>[2x]MPALDLIRPSVTAMRVIASVNADFARELKLPPHIRSLGLISADSDDVTYIAA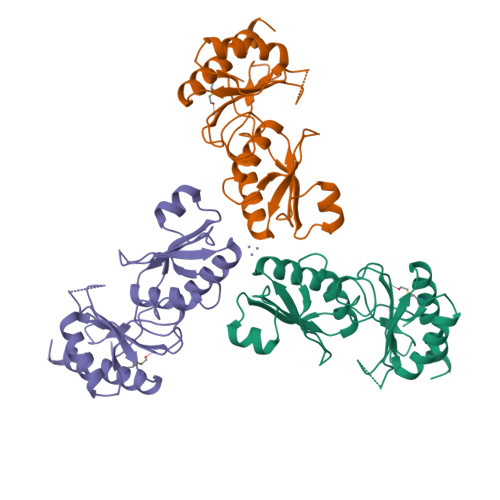DEATKQAMVEVVYGRSLYAGAAHGPSPTAGEVLIMLGGPNPAEVRAGLDAMIAHIENGAAFQWANDAQDTAFLAHVVSRTGSYLSSTAGITLGDPMAYLVAPPLEATYGIDAALKSADVQLATYVPPPSETNYSAAFLTGSQAACKAACNAFTDAVLEIARNPIQRAHHHHHH>[2x]GHMNANLPPSAISELHGPRLLLRAWRDSDREAFAEMCADPQVMEFF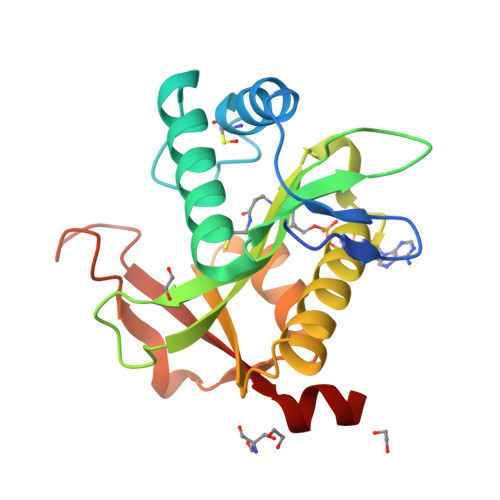PSVLDRAQSDALVDRVQAHFAERGYGPWALELPGEAAFIGFTGLFDVTMDVHFAPTVEIGWRLAPAYWGRGLAREAAETALDFAFERLRLPEVVAFTTPPNRRSWGLMERLGMRRDPAEDFDHPLLAADHPMRRHILYRVDAARWAER> XV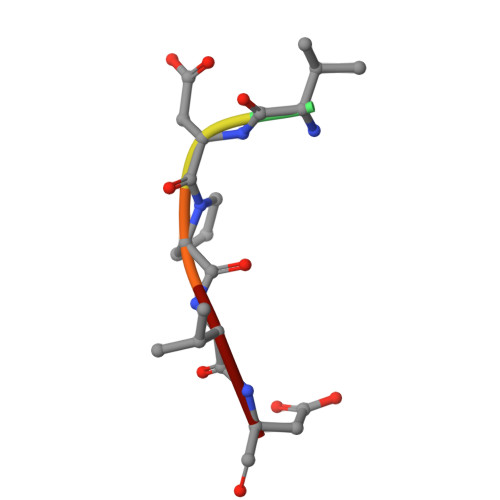DPVD>[2x]GIDPFTSTQTAEDKEEPLHSIISSTESVQGSTSKHEFQAETKKLLDIVARSLYSEKEVFIRELISNASDALEKLRHKLVSD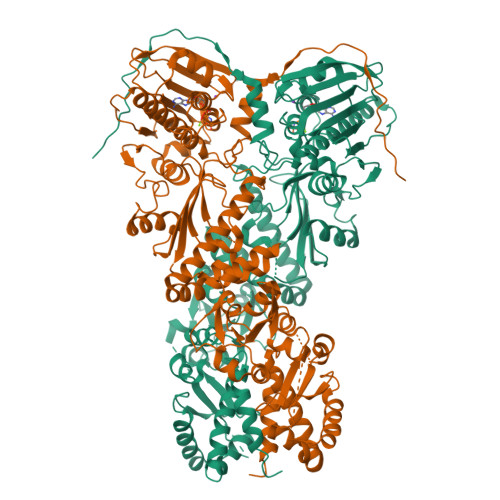GQALPEMEIHLQTNAEKGTITIQDTGIGMTQEELVSNLGTIARSGSKAFLDALQNQAEASSKIIGQFGVGFYSAFMVADRVEVYSRSAAPGSLGYQWLSDGSGVFEIAEASGVRTGTKIIIHLKSDCKEFSSEARVRDVVTKYSNFVSFPLYLNGRRMNTLQAIWMMDPKDVGEWQHEEFYRYVAQAHDKPRYTLHYKTDAPLNIRSIFYVPDMKPSMFDVSRELGSSVALYSRKVLIQTKATDILPKWLRFIRGVVDSEDIPLNLSRELLQESALIRKLRDVLQQRLIKFFIDQSKKDAEKYAKFFEDYGLFMREGIVTATEQEVKEDIAKLLRYESSALPSGQLTSLSEYASRMRAGTRNIYYLCAPNRHLAEHSPYYEAMKKKDTEVLFCFEQFDELTLLHLREFDKKKLISVETDIVVDHYKEEKFEDRSPAAECLSEKETEELMAWMRNVLGSRVTNVKVTLRLDTHPAMVTVLEMGAARHFLRMQQLAKTQEERAQLLQPTLEINPRHALIKKLNQLRASEPGLAQLLVDQIYENAMIAAGLVDDPRAMVGRLNELLVKALERH> DSRKTYTLTDYLKNTYRLKLYSLRWISDHEYLYKQENNILVFNAEYGNSSVFLENSTFDEFGHSINDYSISPDGQFILLEYNYVKQWRHSYTASYDIYDLNKRQLITEERIPNNTQWVTWSPVGHKLAYVWNNDIYVKIEPNLPSYRITWTGKEDIIYNGITDWVYEEEVFSAYSALWWSPNGTFLAYAQFNDTEVPLIEYSFYSDE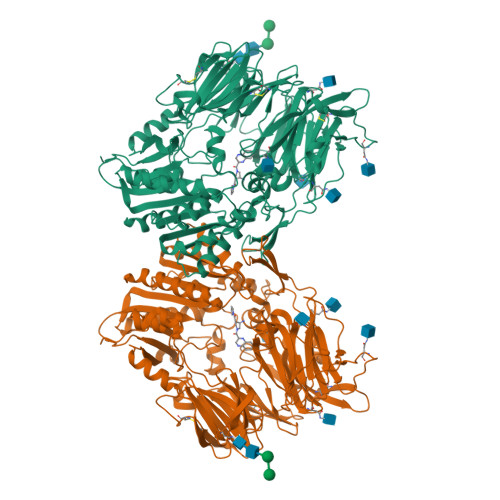SLQYPKTVRVPYPKAGAVNPTVKFFVVNTDSLSSVTNATSIQITAPASMLIGDHYLCDVTWATQERISLQWLRRIQNYSVMDICDYDESSGRWNCLVARQHIEMSTTGWVGRFRPSEPHFTLDGNSFYKIISNEEGYRHICYFQIDKKDCTFITKGTWEVIGIEALTSDYLYYISNEYKGMPGGRNLYKIQLSDYTKVTCLSCELNPERCQYYSVSFSKEAKYYQLRCSGPGLPLYTLHSSVNDKGLRVLEDNSALDKMLQNVQMPSKKLDFIILNETKFWYQMILPPHFDKSKKYPLLLDVYAGPCSQKADTVFRLNWATYLASTENIIVASFDGRGSGYQGDKIMHAINRRLGTFEVEDQIEAARQFSKMGFVDNKRIAIWGWSYGGYVTSMVLGSGSGVFKCGIAVAPVSRWEYYDSVYTERYMGLPTPEDNLDHYRNSTVMSRAENFKQVEYLLIHGTADDNVHFQQSAQISKALVDVGVDFQAMWYTDEDHGIASSTAHQHIYTHMSHFIKQCFSLP>[3x]TSDDHVPVDITDLLDRAAHDAARIYPDLDVSLVPSPTCIIVGLPAGLRLAVDNAIANAVKHGGATLVQLSAVSSRAGVEIAIDDNGSGVPEGERQVVFERFSRGSTASHSGSGLGLALV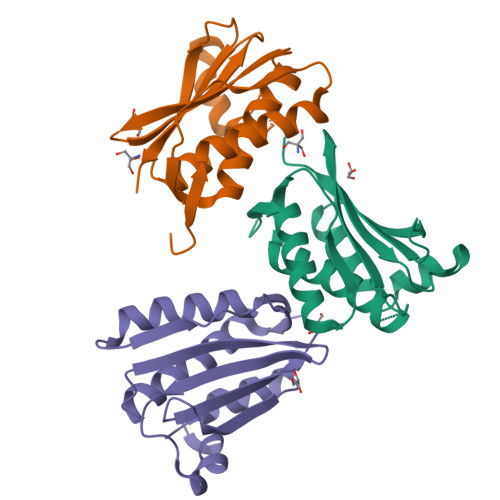AQQAQLHGGTASLENSPLGGARLVLRLPGPS(3S)-3-hydroxy-2,3-dihydro-1H-indole-5,6-dione 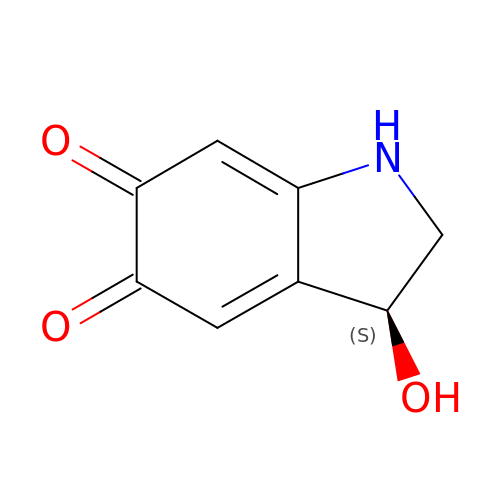| C8 H7 N O3 | LXXQZMIOKXLXPT-MRVPVSSYSA-N> MCSSINEGPYNSPTFGKSLSLKVDGGFNAVSINPSGRDIVLASRQGLYIIDLDDPFTPPRWLHHITPWQVADVQWSPHPAKPYWIVSTSNQKAIIWNLAKSSSNAIEFVLHGHSRAITDINFNPQHPDVLATCSVDTYVHAWDMRSPHRPFYSTSSWRSAASQVKWNYKDPNVLASSHGNDIFVWDLRKGSTPLCSLKGHVSSVNSIDFNRFKYSEIMSSSNDGTVKFWDYSKSTTESKRTVTTNFPIWRGRYLPFGEGYCIMPMVGGNNAVYLINLCDDDDSEQNKKTKLQPIYAFKGHSDRVIDFLWRSRHTCDGDYDDREFQLVTWSKDCDLKLWPISDSIYGKVNFDRGKRLEEKLPDYDYCSYNKEPENRENVQKNEFRRLRENFVTTSGLKKNKTNHITWLSGIRMNSATSQEDLFNETKIQNLGEEVSAIGHKFPKVVFEKISVSTRELCLTLNGPWSEENPDDYIFLRISINFPLNYPNKGDPPKFTIEENSNLTMSKRQEILSNLATIGQKYTDSNLYCLEPCIRFVLGEKVSLEDIEEGQEPLLNFDIADHIDFEELSSLDSSYSDSQNPENLSSQSDIESYKEALVFPDTSNQGLDFGRNLALDTTPVPNGCGSCWTATGELFCFFANEKKPEKKQNAIIKLSQKEAGVEKHPFKIEPQVLYDKEVDSSVITAADELKARPKRYVDTLGLGGGTNGDSRTYFDDETSSDDSFDSVADDWDDILRNDIIVRTKIPILRGNFKAFSSVHSESGKTVESTKKNKNLVISKNFSSLLSDRKELALEYLFMDATPEGFARNNALVAEKFDLDEISHCWQILSDMLIDQSDYDPYTTIWNNHPMGIKWFIKEAIVYFERQQNLQMLAMLCCVILSARRKKIPARYYGQELENMEGTIVFNDNESQNTSFWKGSDAFSTRSRSSTVTPNFYGNHLRGKNIHGGDNSSIRSDDHHARLRTHNTLNGSSKFTEPAQKQGSRAISSSPFHSRMPDIKVELLHDDIIEAYEQEDLLHLEVSDIPKFQTYIYQYSKLLFRWGLPLERVKILKVSTDFRSSYSSQGIPPNNNKKSPYNGVLTHWIENNEFGEEKFLARNCNYCDLRVTRSSFICGNCQHVLHSSCARIWWEIGDECPSGCGCNCPEMFDA;> MLSYFQGFVPIHTIFYSVFHPTEGSKIKYEFPPNNLKNHGINFNTFKNYIIPKPILCHKLITFKYGTYRIVCYPVTINSPIYARNFFSFNFVFVFPYDCETSPYEPAITRLGKMFKVLEEQNQLLSKSERDPVFFDLKVLENSTTTPSTAGPSSTPNPSSNTTPTHPTSEKDTKDMRSSRYSDLIKDLGLPQSAFSIQDLLMRIFQDLNNYSECLIPIDEGNAVDIKIFPLLRPPTTCVSLEDVPLSSVNLKKIIDVNWDPTMMSIVPYIDGLNSIAKISKLSNSDPGLVIECIRHLIYYKCVTLSDIFQFSNIYAPSSLIRNFLTDPLMASDCQSYVTFPEVSKISNLPLNKSLGSGDQDSPSFSVRRKSKSSSIPSNPDSRTTSFSSTSRVSQNSSLNSSFSSIYKDWRQSQTSCSSSNIHVINNRNRFLPTRSCLFDLYRSLSQGQTLKTWYESKYMILKENNIDIRRFITFGLEKRIIYRCYSFPVMINAGSREPKEMTPIITKDLVNNDKLLEKRNHNHLLSATGSRNTAQSGNLKPERPSKVSFEMQRVSSLATGKSTMPKLSDEEEGILEESIRNAETFDKICVLLSKPKLEVESYLNELGEFKVINS;> MDECLPNSCLLGVHLVISTHSGPQIVYHYPPSNTAFLTNNPTKHQHLYGNHANLNKNTSTNKEEKLFNSGSTKTASQIALNESAKSYNTAITPSMTNTNTNNVTLPPTRSHANTVGSQSSIPAATNGVGYRKTDIEDTSRTFQYQETESETSSSGLSDSELSTDYLDISSDSFSISSSLSSSSLSSSPSSSSSSSPPQDGLSRTNSSFQSTDSMSPTSPQMIMENDSISVAESYLDSGTNNKSRAASKRSQNFFHKLSTKKSTDSKTHSPVRKLKSKPSQSTKKGNKLLKNTSNETDGNAFTGSCSISSKKSLSSTGEHNQELRNSSLNDTPGQSPHHYHHRYHHYHKNAATSQRNSHTQYDVEEEDMEVSAMLQDGKISMNEIFFEEENFQDINKILEFDNDFVAEFCSPEREMCNTRFEFTVDNFCFLGLPIHVDSQGRWRKSKHKNKTRSKRSSSTTTNISRKKSIASKISSLSENTLKKVNSGEADTVYDSNIGHEASTDTPNLRINTDVSGNEFEREKEDLGKNMNMFHVCFVMNPHLIEYNKRIDDMYQFVVTRLSLLLRYVQSKTSYISSECHIILKEKERVLKHSKTYQSIRGAGNKGKYLYQRILAKSSLARALTECVDKIQRNEIACLEINDDKVISLQIPIQNEFEKMPNFKLQPVLRGSYLTSILNMKFLEKSSLRIESQNRQNDQAQFSDTNNNIYRFGNNINSTGHCGAANVDDGDDNESNYYCDDNDDLLNYALLLLDEPNNIISSLETFSYQDDIGTIILKHLVRNIQPNIPLRSYRYLITDLLDNPSSLDDLTTETNSLESSILRSCALHLMYWRHARIVIPLSSKYTYIVSPLAPIQGYTIDDYKSTSQNDGNVKKMDDRENNKSGSDRVPLIYQNSMLFRSKFPSLPSLPIFLSLLSTDKPQAYSNIIPSREHKPVYLNALAWLIQYGYVTQLLTFINIRVDKHIKMAVDEDLEKEGFRKTNTARRPSMDYKKTDKKLDDEDGQSRDANASEACSGKNEGMQSNDNNKDVDEKDNENDSRVDDRDDNEIAIADEEEILHFEYDDPEMQHDYTIILEPERATAIEKRWLYRCIYGQPSDIQILFNKLLKYFNGKVPMELVIIKEEISRHDLKKLLNALDKYLIEIHHW;> MFAKLHGKKQRPISSINSQTPRTSNTTHANSISLSSGNLIVGSNRNLRQKKEQFGSQQRASGRKLISNKENDDNVNNGGDNNYDNGERVHRHHIPGLKIKAYQAELGYHESRFSENLVMLNLVEFPDIKPGDLVELKTYHKNPSASNGDKKIYFIAKDFDGETKRRAKTSNVSILSGQLQTLLDLPSRSRIWIKLKPNKFDLQADVVEFNIKDCLLNRGDMWVLSSKLVDTCVFMDQRLAFLDSIRGTIKGIYRNGKKIVSGYIGEQTRIIFRSESARLIFLIQITDEMWNFEETGEQLFQKMVNSFFPKIFKKWKDVDTHHTITIAFAISMDLSDTSFKDLTPGESLKNSQDYFRIVVDQVSIIHWVDIMETLREEFMEIRKDLLNKQTDKGYSVANGRFSPVIKSNFLELVNFATTILTDPFKQLDLRHTTTHVMIISPGSGLFDVDYSLLRLTGKKLLSLEMTMDLICLSKAPLHIVPLFRYRDFENKLHHCVPLWLSVFFWNDHDKKSNSEWTPRCKIYDLQMMGITENELIREVDVEYLQLNKKVKSLSEFMNDYDKNAFEVKILCAGSNTKQSKKLNSKFDTVFENDVVVKARKIPATATTTHGNTKFIWRGPKVALPAIKDIQKPNVIPDLSIKTIEASFYDDCNTTNDKISTPTTSNNDNLEMNDSLVSVRSADNQNTSLALDSLKGLSKRNSLKDFTQRVITKFISNIDTSKNKKIKSTLLRDDVDNSPLGSNTPLPSSESKISGLKLQQKGLADENVISKRGNLIIKKNLSIFGLPSNEIMSGSPSSYLGSSHTRTSSKLSNMSDKAAFITEGQKSKHDDSNTYSLTQQLKHRISETWVDIKSPSIPVSSEFANELLPIRWKDVWPKYVARKYSKWRSFTTPAELPITISDFPSKDDFDRNFIFRNHSVTLNTDQEQYNQTYKDLLRDMIYMRLLTGFQICVGRQVEKIELSRESGESETVVNKYLDFNQNDAFKLYLMIDSEIHRITCSSSGIIDVERYLRKDEANLFDQVPSYIPLVKTRYESSFRDAMIDPLHVKRESLNWNQIDQVLAGYGDNLIDRKWHGFRAKYVVLPTDIPPNTYSMVINGKSETLNPEEIRVEGLRRLIGSITRSRLRTEKEKKGRKTKREEIQPEVMFYTGPLYNFINEQQTSLESSAINFKDSIFVNDNNLLNRNVELSKLAYQIQRGEDRITLVNRKWHWKKHEKCFVGSEMVNWLIRNFSDIDTREDAIKYGQKVMKEGLFVHVLNKHNFLDGHYFYQFSPEYVMDTNKLEKTNSHRSTLSDPKQMLRKASTGSSNDPSAMTPFSSVVPAISASNASVADAKEPSRPILMLSNSLVIDVDPAGKSSKQESCTVHYDRVHNPDHCFHIRLEWLTTTPKLIDDLVGNWSRLCERYGLKMIEIPWEELCTIPSVNPFHSFVEIKLAINPWEDPEFKDRELFAKSKFYYHVYLLKASGFLLDNRASKFLQNQDIEFDIMYSWGKPQFKYVQYIHHTGAYVAELRENGCLFLAPNNIYISRVNPGNIIGKIHSASSSSLDAQKVILNFKSTCLDYQKLRSIFLDAKEMWITGKIVED

The SEA complex (SEAC) is a growth regulator that acts as a GTPase-activating protein (GAP) towards Gtr1, a Rag GTPase that relays nutrient status to the Target of Rapamycin Complex 1 (TORC1) in yeast. Here, we solve the cryo-EM structure of the native eight-subunit SEAC. The SEAC has a modular structure in which a COPII-like cage corresponding to SEACAT binds two flexible wings, which correspond to SEACIT. The wings are tethered to the core via Sea3, which forms part of both modules.

We used a series of masks and focused refinements to improve the resolution, yielding maps at 2.8 Å and 2.7 Å resolution for the core and wings, respectively. Npr2 and Npr3 consist of an N-terminal lobe (N-lobe) and a C-terminal lobe (C-lobe), which interact with each other and are connected via a linker. The N-lobes contain the longin domains and are far from the SEAC core, whereas the C-lobe heterodimer faces the Sea4 β-propeller domain (II or III). As detailed below, the Npr2N-lobe also contains the catalytic arginine (Npr2Arg84). Sea1 is positioned at the edge of the wing and uses its SABA domain to interact with Npr2, whereas the C-terminal region (Sea1Cter), comprising the SHEN, the DEP (which is not resolved) and the CTD, is more flexible and does not interact with the rest of the wing. We could resolve an extension in the Sea1SABA that becomes partially ordered and inserts between the Sea3SIP β-propeller and the Npr2C-lobe, interacting with and wrapping the latter. The interaction between Sea1 and Npr2 appears to be stabilized by the Sea3SIP, as its β-propeller is positioned on top of the Sea1SABA–Npr2N-lobe junction, forming a tripartite Sea1–Npr2–Sea3 interaction. The Npr3C-lobe plays an important role in organizing the wing relative to the core, as it is sandwiched between the Sea4 β-propeller and the Sea3 RWD, in addition to contacting the Npr2C-lobe. Npr2Arg84, the GATOR1-equivalent catalytic residue located in the Npr2N-lobe, is solvent accessible and positioned opposite to the core–wing interface, far from any element of the core or the Sea3SIP. Our structure thus predicts that, as in GATOR1, Npr2Arg84 rather than Sea1Arg943 is the catalytic arginine and that the SEAC is in an active conformation (that is, binding of SEACAT to SEACIT is not sufficient to inhibit its GAP activity).>AATYAQTLQNIPETNVTTLDNGLRVASEESSQPTCTVGVWIGAGSRYENEKNNGAGYFVEHLAFKGTKKRPCAAFEKEVESMGAHFNGYTSREQTAFYIKALSKDMPKVVELLADVVQNCALEESQIEKERGVILQELKEMDNDMTNVTFDYLHATAFQGTALARTVEGTTENIKHLTRADLASYIDTHFKAPRMVLAAAGGISHKELVDAARQHFSGVSFTYKEDAVPILPRCRFTGSEIRARDDALPVAHVALAVEGPGWADPDNVVLHVANAIIGRYDRTFGGGKHLSSRLAALAVEHKLCHSFQTFNTSYSDTGLFGFHFVADPLSIDDMMFCAQGEWMRLCTSTTESEVKRAKNHLRSAMVAQLDGTTPVCETIGSHLLNYGRRISLEEWDSRISAVDARMVRDVCSKYIYDKCPALAAVGPIEQLLDYNRIRSGMYWIRF[2x];>[2x]SLKVAPKVAVSAAAERVKLCPGAEDLEITKLPNGLIIASLENFSPASRIGVFIKAGSRYETTANLGTAHLLRLASPLTTKGASSFRITRGIEAVGGSLSVYSTREKMTYCVECLRDHVDTVMEYLLNVTTAPEFRPWEVTDLQPQLKVDKAVAFQSPQVGVLENLHAAAYKTALANPLYCPDYRIGKITSEQLHHFVQNNFTSARMALVGIGVKHSDLKQVAEQFLNIRSGAGTSSAKATYWGGEIREQNGHSLVHAAVVTEGAAVGSAEANAFSVLQHVLGAGPLIKRGSSVTSKLYQGVAKATTQPFDASAFNVNYSDSGLFGFYTISQAAHAGEVIRAAMNQLKAAAQGGVTEEDVTKAKNQLKATYLMSVETAQGLLNEIGSEALLSGTHTAPSVVAQKIDSVTSADVVNAAKKFVSGKKSMAASGDLGSTPFLDEL;>MAPNIRKSHPLLKMINNSLIDLPAPSNISAWWNFGSLLAVCLMTQILTGLLLAMHYTADTSLAFSSVAHTCRNVQYGWLIRNLHANGASFFFICIFLHIGRGLYYGSYLYKETWNTGVILLLTLMATAFVGYVLPWGQMSFWGATVITNLFSAIPYIGHTLVEWAWGGFSVDNPTLTRFFALHFLLPFAIAGITIIHLTFLHESGSNNPLGISSDSDKIPFHPYYSFKDILGLTLMLTPFLTLALFSPNLLGDPENFTPANPLVTPPHIKPEWYFLFAYAILRSIPNKLGGVLALAASVLILFLIPFLHKSKQRTMTFRPLSQTLFWLLVANLLILTWIGSQPVEHPFIIIGQMASLSYFTILLILFPTIGTLENKMLNY[2x];>GELELHPPAFPWSHGGPLSALDHSSVRRGFQVYKQVCSACHSMDYVAFRNLIGVTHTEAEAKALAEEVEVQDGPDENGELFMRPGKISDYFPKPYPNPEAARAANNGALPPDLSYIVNARHGGEDYVFSLLTGYCDPPAGVVVREGLHYNPYFPGQAIGMAPPIYNEILEYDDGTPATMSQIAKDVCTFLRWAAEPEHDQRKRMGLKMLLISALLTSLLYYMKRHKWSVLKSRKMAYRPPK[2x];>[2x]VHNDVTVPDFSAYRREDVMDATTSSQTSSEDRKGFSYLVTATACVATAYAAKNVVTQFISSLSASADVLALSKIEIKLSDIPEGKNVAFKWRGKPLFVRHRTQAEINQEAEVDVSKLRDPQHDLDRVKKPEWVILVGVCTHLGCVPIANSGDFGGYYCPCHGSHYDASGRIRKGPAP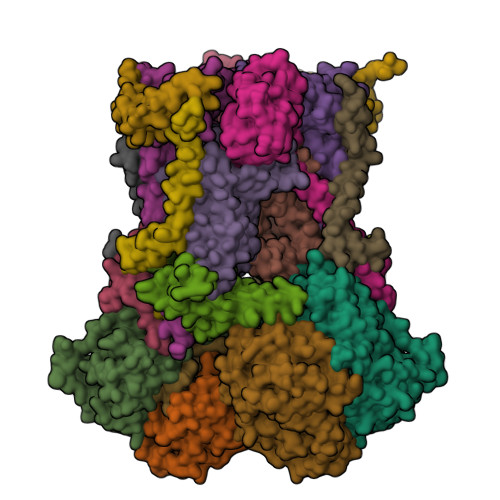YNLEVPTYQFVGDDLVVVG;>[2x]AARATVAGGGRLMDRIRKWYYNAAGFNKYGLMRDDTLYEDDDVKEALKRLPEDLYNERMFRIKRALDLSLKHRILPKEQWVKYEEDKPYLEPYLKEVIRERLEREAWNKK;>[2x]GIHFGNLARVRHIITYSLSPFEQRAIPNIFSDALPNVWRRFSSQVFKVAPPFLGAYLLYSWGTQEFERLKRKNPADYENDQ;>[2x]LRGSGEEEEEELVDPLTTIREHCEQTEKCVKARERLELCDARVSSRSHTEEQCTEELFDFLHARDHCVAHKLFNKLK;>ALLRQAYSALFRRTSTFALTVVLGAVLFERAFDQGADAIFEHLNEGKLWKHIKHKYEASEE[2x]>[2x]MRGSHHHHHHGSMPDLLTNVAENYVNQDLFAGIEWRIDQDGKPIFQGCAGVKDIETRTF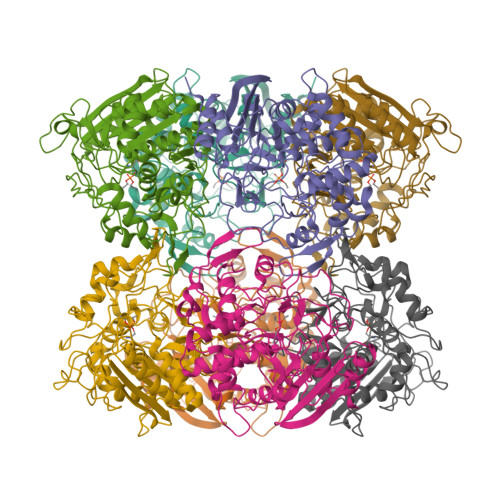IPKNAIYRIYSMTKPIVSFLAMMLIERGVFRLSSPIQNFDPRFKSMKVIDQHAHIEPATALITIEHLLTHQAGFSYDFSLGCPISAHYRDAQLIEDGGRDLTDMMGVLAELPLVFHPGTQWKYSISTDVLAHIIECATGERVDDLLQRLIFDPLDMQDTGFSLPLDGASRLMEVYGMRSLHGLPALKPAPHVLVPADLGSSHPTDDPDFRRGGHGLYSTLDDYMAFANMLLSGQTPEGETLLSPAVLKLALAPRVHFGARGMRINDEPFAGYSWNLLGRVMTDVGAAAYATHLGEFGWSGAAATYFWVDPTKNMTGCVMTQFLGSQHPIGSDMQAAAMSMLG>MMGRGKLILIEGLDRTGKTTQCNILYKKLQPNCKLLKFPERSTRIGGLINEYLTDDSFQLSDQAIHLLFSANRWEIVDKIKKDLLEGKNIVMDRYVYSG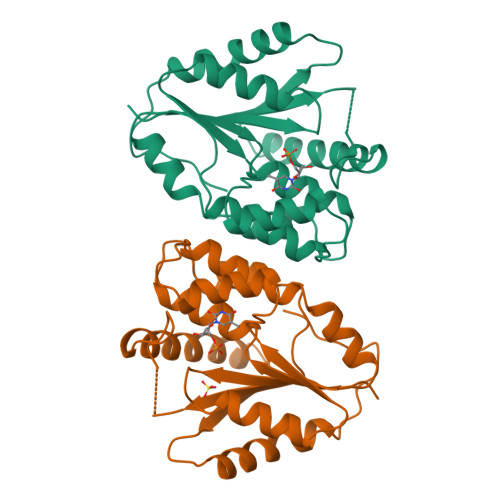VAYSAAKGTNGMDLDWCLQPDVGLLKPDLTLFLSTQDVDNNAEKSGFGDERYETVKFQEKVKQTFMKLLDKEIRKGDESITIVDVTNKGIQEVEALIWQIVEPVLSTHIDHDKFSFF[2x]>MGHSSSDPVYPCGICTNEVNDDQDAILCEASCQKWFHRICTGMTETAYGLLTAEASAVWGCDTCMAD[2x];>[2x]AMAAKVVYVFSTEMANK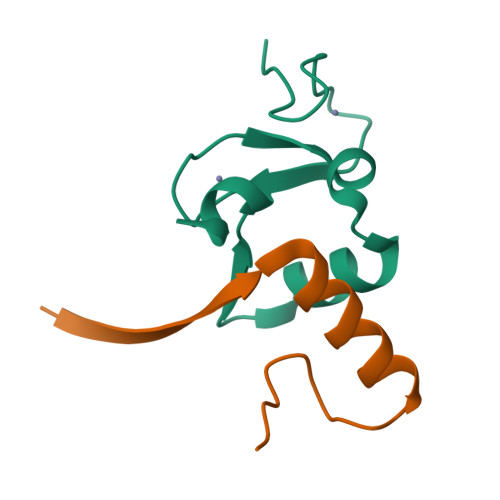AAEAVLKGQVETIVSFHI> GSHMTRETIFEASKKV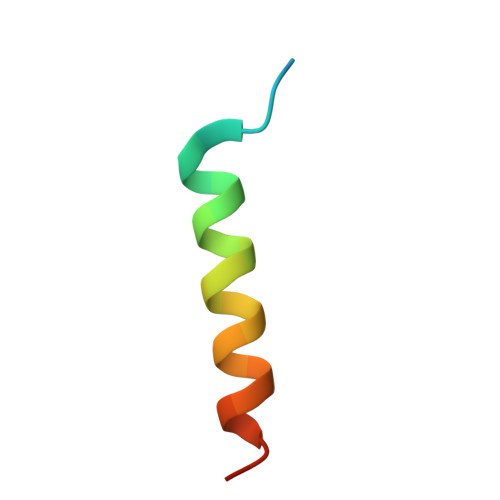TNSLSNLISLIGT> G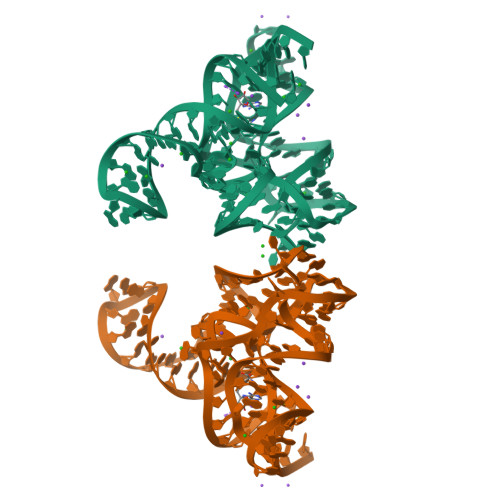GCUUAUCAAGAGAGGGCAAGAGACUGGCUUGAUGACCCCCGGCAACCAAAAAUGGUGCCAAUUCCUGCAGAGGAAACGUUGAAAGAUGAGCCA Aminoacyl t-RNA synthetases (aaRS) are ligases that conjugate a t-RNA with the cognate amino acid to ensure protein biosynthesis in the ribosome. The enzymatic reaction consists of a two-step process, the first involving the formation of aminoacyladenosine, and the second featuring the transfer of the amino acid from this reactive intermediate to the cognate t-RNA. Threonyl t-RNA synthetase (ThrRS) is one of the enzymes involved in this pathway, and it has been validated as an anti-malarial drug target. Here, we present 9 structurally diverse low micromolar Plasmodium falciparum ThrRS inhibitors that were identified using high-throughput virtual screening (HTVS) and were verified in a FRET enzymatic assay.

Attempts were made to co-crystallise these inhibitors with PfThrRS to enable experimental structure-based drug design; however, no crystals suitable for X-ray analysis were obtained for the Plasmodium falciparum ThrRS isoform. Since crystallisation condition protocols for the E. coli ThrRS were available, and since the ThrRSs of the two organisms share 94.7% sequence identity in the binding site (within 3 Å from ThrAMS; 89.2% within 5 Å; see binding site sequence alignment in Fig 14A), attempts were made to co-crystallise the identified inhibitors with the EcThrRS, and use this information to guide compound optimisation. Crystallisation experiments resulted in the determination of the crystal structure of the EcThrRS-7q complex, which was resolved at 2.08 Å resolution. Structure analysis confirmed the docking predictions that the compound binds in a threonine-binding subsite and that the salicylic acid hydroxyl and carboxylic groups coordinate the zinc ion (the heavy atom RMSD value between the crystallised and docked pose is 2.54 Å). The binding mode of the zinc-coordinating phenol/carboxylic acid group was identical when comparing the experimental crystal structure and the docked model. However, there were minor differences in the conformation of the sulphonamide group. The sulphonamide group was slightly twisted with respect to the docked pose, and besides binding to Arg651, it simultaneously forms interactions also with Lys752, Gln766 and Gln 771. The discrepancy between the binding mode of the resolved and the docked sulphonamide group was the result of Lys752, Gln766 and Gln 771 side chain mobility, as the conformations showed by these residues were different from those in the complex with ThrAMS. Structure-activity relationship study was supported by the crystal structure of the complex of a salicylic acid analogue with a close homologue of the plasmodium target, E. coli ThrRS (EcThrRS). Despite the availability of the structural information on the ligand binding mode, targeted incorporation of hydrogen bond donors and acceptors to mimic the adenine of the substrate did not yield compounds with substantially improved potency.

>[2x]DHRKIGKQLDLYHMQEEAPGMVFWHNDGWTIFRELEVFVRSKLKEYQYQEVKGPFMMDRVLWEKTGHWDNYKDAMFTTSSENREYCIKPMNCPGHVQIFNQGLKSYRDLPLRMAEFGSCHRNEPSGSLHGLMRVRGFTQDDAHIFCTEEQIRDEVNGCIRLVYDMYSTFGFEKIVVKLSTRPEKRIGSDEMWDRAEADLAVALEENNIPFEYQLGEGAFYGPKIEFTLYDCLDRAWQCGTVQLDFSLPSRLSASYVGEDNERKVPVMIHRAILGSMERFIGILTEEFAGFFPTWLAPVQVVIMNITDSQSEYVNELTQKLSNAGIRVKADLRNEKIGFKIREHTLRRVPYMLVCGDKEVESGKVAVRTRRGKDLGSMDVNEVIEKLQQEIRSRSLKQLEE N-[(4-aminophenyl)methyl]adenosine | C17 H20 N6 O4 | 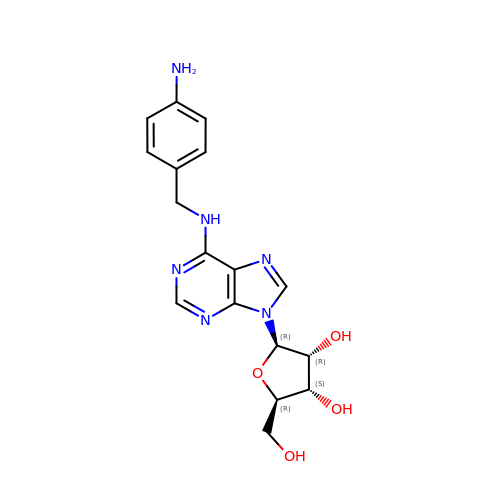PMUVNAUPWLXPSA-LSCFUAHRSA-N>[8x]MSVSAFNRRWAAVILEALTRHGVRHICIAPGSRSTLLTLAAAENSAFIHHTHFDERGLGHLALGLAKVSKQPVAVIVTSGTAVANLYPALIEAGLTGEKLILLTADRPPELIDCGANQAIRQPGMFASHPTHSISLPRPTQDIPARWLVSTIDHALGTLHAGGVHINCPFAEPLYGEMDDTGLSWQQRLGDWWQDDKPWLREAPRLESEKQRDWFFWRQKRGVVVAGRMSAEEGKKVALWAQTLGWPLIGDVLSQTGQPLPCADLWLGNAKATSELQQAQIVVQLGSSLTGKRLLQWQASCEPEEYWIVDDIEGRLDPAHHRGRRLIANIADWLELHPAEKRQPWCVEIPRLAEQAMQAVIARRDAFGEAQLAHRICDYLPEQGQLFVGNSLVVRLIDALSQLPAGYPVY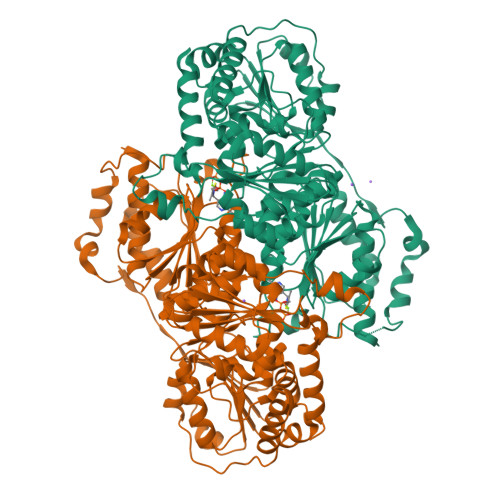SNRGASGIDGLLSTAAGVQRASGKPTLAIVGDLSALYDLNALALLRQVSAPLVLIVVNNNGGQIFSLLPTPQSERERFYLMPQNVHFEHAAAMFELKYHRPQNWQELETAFADAWRTPTTTVIEMVVNDTDGAQTLQQLLAQVSHL[(2R)-4-(2-azanyl-6-oxidanylidene-3H-purin-9-yl)-2-(hydroxymethyl)butyl] dihydrogen phosphate | C10 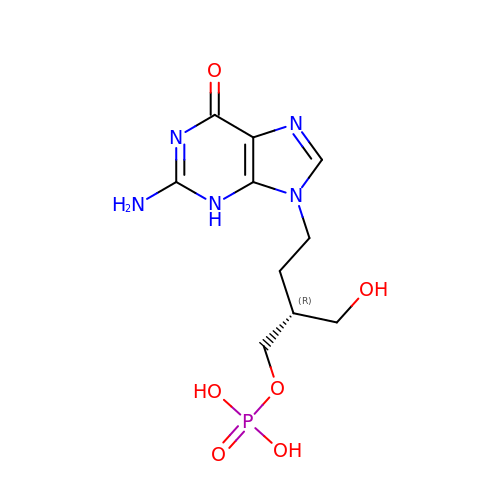H16 N5 O6 P | BLURMGIBVBRPQT-ZCFIWIBFSA-N> MNRIKVAILFGGCSEEHDVSVKSAIEIAANINKEKYEPLYIGITKSGVWKMCE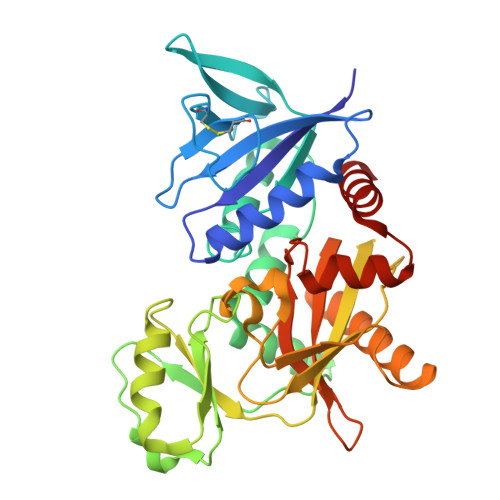KPCAEWENENCYSAVLSPDKKMHGLLVKKNHEYEINHVDVAFSALHGKSGEDGSIQGLFELSGIPFVGCDIQSSAICMDKSLTYIVAKNAGIATPAFWVINKDDRPVAATFTYPVFVKPARSGSSFGVKKVNSADELDYAIESARQYDSKILIEQAVSGCEVGCAVLGNSAALVVGEVDQIRLQYGIFRIHQEVEPEKGSENAVITVPADLSAEERGRIQETVKKIYKTLGCRGLARVDMFLQDNGRIVLNEVNTLPGFTSYSRYPRMMAAAGISLPELIDRLIVLALKG>MTENAEKFLWGVATSAYQIEGATQEDGRGPSIWDTFARRPGAIRDGSTGEPACDHYHRYEEDIALMQSLGVGVYRFSVAWPRILPEGRGRINPKGLAFYDRLVDRLLAAGITPFLTLYHWDLPQALEDRGGWRSRETAFAFAEYAEAVARALADRVPFFATLNEPWCSAFLGHWTGEHAPGLRNLEAALRAAHHLLLGHGLAVEALRAAGARRVGIVLNFAPAYGEDPEAVDVADRYHNRYFLDPILGRGYPESPFQDPPPAPILSRDLEAIARPLDFLGVNYYAPVRVAPGTGPLPVRYLPPEGPVTAMGWEVYPEGLYHLLKRLGREVPWPLYITENGAAYPDLWTGEAVVEDPERVAYLEAHVEAALRAREEGVDLRGYFVWSLMDNFEWAFGYTRRFGLYYVDFPSQRRIPKRSALWYR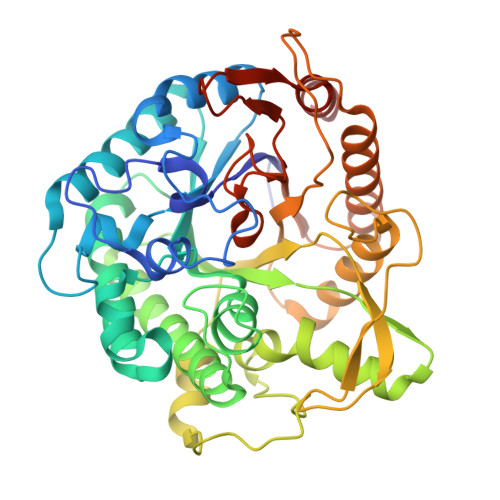ERIARAQTGGSAH[2x]XYLOSE-DERIVED ISOFAGOMINE LACTAM | C5 H9 N O2 | 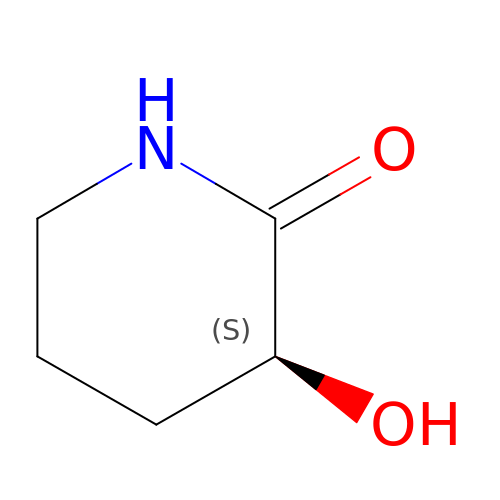RYKLZUPYJFFNRR-BYPYZUCNSA-N>GPHMVKHPLNTAWTLWYTKPAVDKSESWSDLLRPVTSFQTVEEFWAIIQNIPEPHELPLKSDYHVFRNDVRPEWEDEANAKGGKWSFQLRGKGADIDELWLRTLLAVIGETIDEDDSQINGVVLSIRKGGN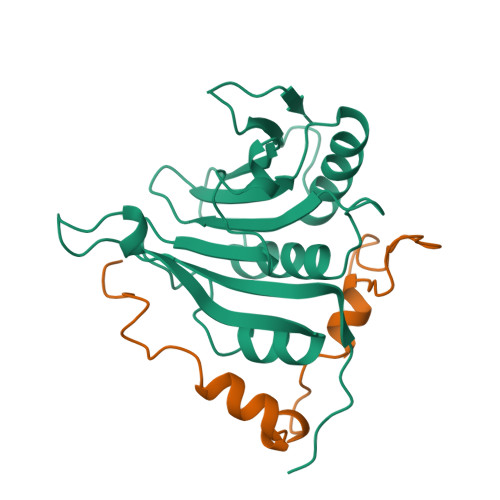KFALWTASEDKEPLLRIGGKFKQVLALTDDGHLEFFPHSSANGRHPQPSITL[2x];>GPHMTDPITNYKPMDLQYKTYAYSMNELYHLKPSLASASYEEDPLISELVRSLPKRKFWRLRMG[2x]Herpes simplex virus type-1 expresses a heterodimeric Fc receptor, gE-gI, on the surfaces of virions and infected cells that binds the Fc region of host immunoglobulin G and is implicated in the cell-to-cell spread of virus. gE-gI binds immunoglobulin G at the basic pH of the cell surface and releases it at the acidic pH of lysosomes, consistent with a role in facilitating the degradation of antiviral antibodies. HSV-1 gE-gI is a heterodimer composed of two type I membrane glycoproteins: gE, a 530-residue protein including a ˜401-residue extracellular region followed by a predicted single transmembrane helix and a ˜106-residue C-terminal cytoplasmic tail; and gI, a 370-residue protein including a ˜248-residue extracellular portion followed by a predicted single transmembrane helix, and a ˜94-residue C-terminal cytoplasmic tail. Here we report the structures of CgE, an Fc-binding fragment of the HSV-1 Fc receptor gE-gI, and a gE-gI complex with Fc.

Here we identify the C-terminal domain of the gE ectodomain (CgE) as the minimal Fc-binding domain and present a 1.78-Å CgE structure. The first and second β-sheets in CgE, which correspond to their counterparts in Ig V domains, contain strands A, B, B′, E, and D, and strands A′, G, F, C, C′, and C′′, respectively. The CgE fold lacks the disulfide bond that joins the A′GFCC′C′′ and the DEBB′A sheets in the canonical Ig fold, with CgE containing a cysteine in strand F (Cys359) but a valine in the complementary position in strand B (Val244). However, the conserved tryptophan normally found in strand C adjacent to the intersheet disulfide bond is present in CgE (Trp262). Even within the region of CgE that resembles an Ig V domain, CgE has a different disulfide-bonding pattern and is longer and more open than others in the Ig superfamily. Differences between the pIgR and CgE Ig V folds include the positions of the CDR loops, the predicted Fc-binding sites (described for CgE below), the overall size, with CgE being larger due to its extended strands C, C′, and C′′, and the third β-sheet in CgE, which is absent in pIgR domain 1. However, the structures of CgE and a gE-gI/Fc complex reported here can be used to identify which insertions are likely to disrupt the CgE structure and which insertions are likely to affect function. The structural effects of insertions after gE positions 277 and 291 are difficult to interpret due to their location near disulfide bonds in the third β-sheet of CgE.

>GAPEVSHVRGVTVRMETPEAILFSPGETFSTNVSIHAIAHDDQTYSMDVVWLRFDVPTSCAEMRIYESCLYHPQLPECLSPADAPCAASTWTSRLAVRSYAGCSRTNPPPRCSAEAHMEPVPGLAWQAASVNLEFRDASPQHSGLYLCVVYVNDHIHAWGHITISTAAQYRNAVVEQPLDIEGRGHHHHHH[2x]> STQTAEDKEEPLHSIISSTESVQGSTSKHEFQAETKKLLDIVARSLYSEKEVFIRELISNASDALEKLRHKLVSDGQALPEMEIHLQTNAEKGTITIQDTGIGMTQEELVSNLGTIARSGSKAFLDALQNQAEASSKIIGQFGVGFYSAFMVADRVEVYSRSAAPGSLGYQWLSDGSGVFEIAEASGVRTGTKIIIHLKSDCKEFSSEARVRDVVTKYSNFVSFPLYLNGRRMNTLQAIWMMDPKDVREWQHEEFYRY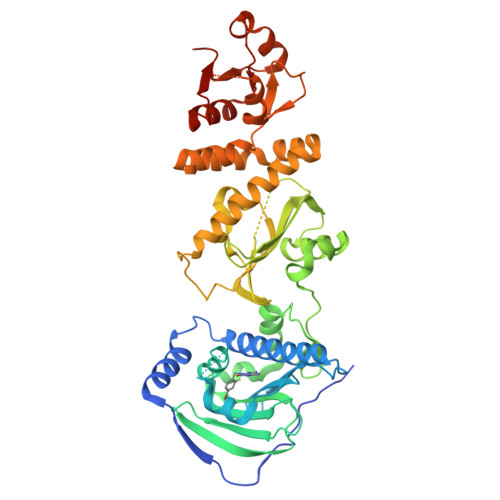VAQAHDKPRYTLHYKTDAPLNIRSIFYVPDMKPSMFDVSRELGSSVALYSRKVLIQTKATDILPKWLRFIRGVVDSEDIPLNLSRELLQESALIRKLRDVLQQRLIKFFIDQSKKDAEKYAKFFEDYGLFMREGIVTATEQEVKEDIAKLLRYESSALPSGQLTSLSEYASRMRAGTRNIYYLCAPNRHLAEHSPYYEAMKKKDTEVLFCFEQFDELTLLHLREFDKKKLISVETDIVVDHYKE> ME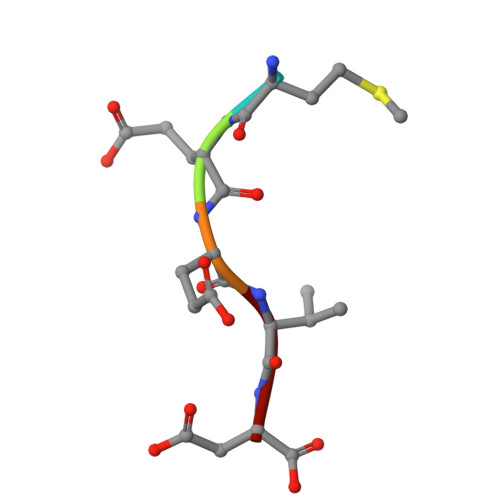EVD7-HYDROXY-4-METHYL-3-(2-HYDROXY-ETHYL)COUMARIN | C12 H12 O4 | 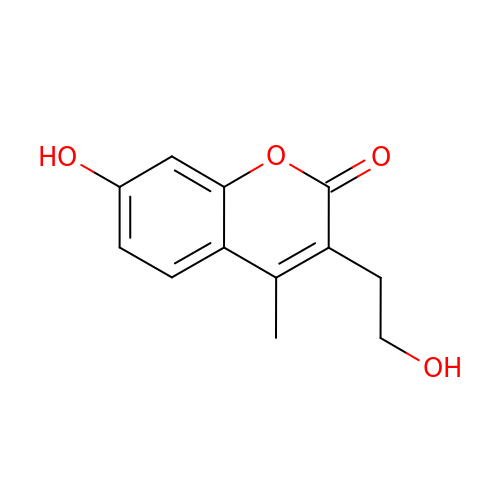VCGFYFKJZGIZMX-UHFFFAOYSA-N Utilizing the published genome sequence of the organism, we hypothesized that the genes 0612, 0638, and 0637 encode for a 4,6-dehydratase, an aminotransferase, and an N-acetyltransferase, respectively, which would be required for the biosynthesis of one of the diacetamido-sugars, 2,4-diacetamido-2,4,6-trideoxy-d-glucose, starting from UDP-N-acetylglucosamine. In this report we present functional and structural data that demonstrate the proteins encoded by the 0638 and 0637 genes do indeed correspond to an aminotransferase (hereafter referred to as Pcryo_0638) and an N-acetyltransferase (Pcryo_0637). In summary, we have demonstrated that the genes in P. cryohalolentis, namely 0638 and 0637, encode for a PLP-dependent aminotransferase and an N-acetyltransferase, respectively. The data presented herein confirm the hypothesized functions of these enzymes and provide new insight into an unusual sugar biosynthetic pathway in Gram-negative bacteria.

The second model of Pcryo_0637 to be determined was that of a ternary complex with UDP-2,4-diacetamido-2,4,6-trideoxy-d-glucose (the product) and CoA. The model was refined to an R-factor of 16.4% at 1.55 Å resolution. The electron density corresponding to the bound ligands is unambiguous. The uracil ring is anchored into the active site by the backbone amide and the carboxylate side chain of Asp 41 and two ordered water molecules. The side chains of Asp 40 and Ser 11, along with a water molecule, lie within 3.2 Å of the ribose hydroxyl groups. Note that the side chain of Ser 11 adopts two conformations, the second of which allows it to form a hydrogen bond with an α-phosphoryl oxygen of the UDP-sugar product. Additionally, the phosphoryl oxygens are surrounded by numerous water molecules and the backbone amide groups of Cys 13 and Ala 75. The pyranosyl group of the UDP-sugar product directly interacts only with the side chain of His 142 and the backbone amide group of Gly 179 (both from a neighboring subunit of the trimer). On the basis of previously determined structures of related N-acetyltransferases, His 142 most likely functions as the active site base.

> GGGHMSKVFAVYGASGCGRSLMPVANEQLRILEGDTDSQIVFIDDALDDNITVNGYTAMNYTKFKSIKNDDKFVLIAIANSSIRQKIADKLVKDGISLWTVQGMTTLIMDEVSIDAGAALSPFVTIAANVTIGKCFHANLYSYVEHDCIIGDYVTFAPRVSCNGNIHIHDHAYIGTGAVIKQGTPDKPLIIGKGAIVGMGAVVTKEVPAGAVVIGNPARLLNK> MITVDITVNDEGKVTDVIMDGHADHGEYGHDIVSAGASAVLFGSVNAIIGLTSERPDINYDDQGGHFHIRSV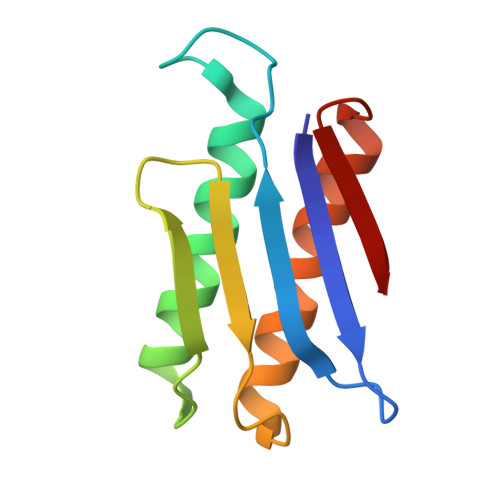DTNNDEAQLILQTMLVSLQTIEEEYNENIRLNYK>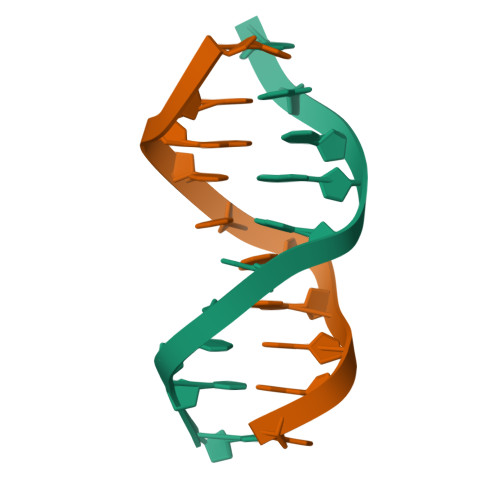CCGCTAGCGG[2x]> NKLTLDKLNVKGKRVVMRVDFNVPMAAAQITNNARIKAAVPSIKFCLDDGAKSVVLMSHLGRPDGSPMPDKYSLQPVAAELKSALGKAVLFLKDCVGPAVEKACADPAAGSVILLENLRFHVEEEGKGKDASGNKAAGEPAKIKAFRASLSALGDVYVNDAFGTAHRAHSSMVGVNLPKKAGAFLMKKELNYFAAAAESPERPFLAILGGAKVADKIQLINNMLDKVNEMIIGGGMAFTFLKVLNNMEIGTSLFDEAGKKIVKNLMSKAAANGVKITLPVDFVTADKFDEQAKIGQATVASGIPAGW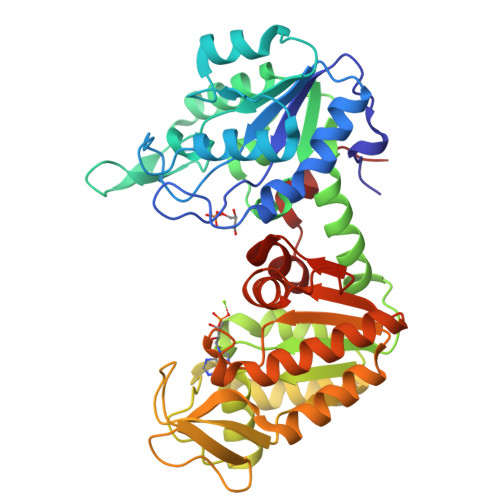MGLDCGPKSSAKYSEAVARAKQIVWNGPVGVFEWEAFAQGTKALMDEVVKATSRGCITIIGGGDTATCCAKWNTEDNVSHVSTGGGASLELLEGKVLPGVDALSNV> VFHKIRNEDLIFNESLGQGTFTKIFKGVRREVGDYGQLHETEVLLKVLDKAHRNYSESFFEAASMMSKLSHKHLVLNYGVCVCGDENILVQEFVKFGSLDTYLKKNKNCINILWKLEVAKQLAWAMHFLEENTLIHGNVCAKNILLIREEDRKTGNPPFIKLSDPGISITVLPKDILQERIPWVPPECIENPKNLNLATDKWSFGTTLWEICSGG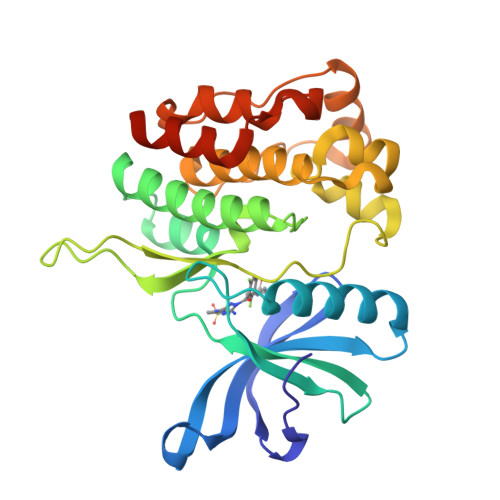DKPLSALDSQRKLQFYEDRHQLPAPKWAELANLINNCMDYEPDHRPSFRAIIRDLNSLFTPDHHHHHH>MLSRKGIIPEEYVLTRLAEDPAEPRYRTRERRARFVSKKGNCNVAHKNIREQGRFLQDVFTTLVDLKWPHTLLIFTMSFLCSWLLFAMVWWLIAFAHGDLAPGEGTNVPCVTSIHSFSSAFLFSIEVQVTIGFGGRMVTEECPLAILILIVQNIVGLMINAIMLGCIFMKTAQAHRRAETLIFSKHAVITLRHGRLCFMLRVGDLRKSMIISATIHMQVVRKTTSPEGEVVPLHQVDIPMENGVGGNGIFLVAPLIIYHVIDSNSPLYDLAPSDLHHHQDLEIIVILEGVVETTGITTQARTSYLADEILWGQRFVPIVAEEDGRYSVDYSKFGNTIKVPTPLCTARQLDEDRSLLDALTLASSRGPLRKRSVAVAKAKPKFSISPDSLS[4x];>MPLAFCGTENHSAAYRVDQGVLNNGCFVDALNVVPHVFLLFITFPILFIGWGSQSSKVHIHHSTWLHFPGHNLRWILTFILLFVLVCEIAEGILSDGVTESRHLHLYMPAGMAFMAAITSVVYYHNIETSNFPKLLIALLIYWTLAFITKTIKFVKFYDHAIGFSQLRFCLTGLLVILYGMLLLVEVNVIRVRRYIFFKTPREVKPPEDLQDLGVRFLQPFVNLLSKGTYWWMNAFIKTAHKKPIDLRAIGKLPIAMRALTNYQRLCVAFDAQARKDTQSPQGARAIWRALCHAFGRRLILSSTFRILADLLGFAGPLCIFGIVDHLGKENHVFQPKTQFLGVYFVSSQEFLGNAYVLAVLLFLALLLQRTFLQASYYVAIETGINLRGAIQTKIYNKIMHLSTSNLSMGEMTAGQICNLVAIDTNQLMWFFFLCPNLWAMPVQIIVGVILLYYILGVSALIGAAVIILLAPVQYFVATKLSQAQRSTLEHSNERLKQTNEMLRGMKLLKLYAWESIFCSRVEVTRRKEMTSLRAFAVYTSISIFMNTAIPIAAVLITFVGHVSFFKESDLSPSVAFASLSLFHILVTPLFLLSSVVRSTVKALVSVQKLSEFLSSAEIREEQCAPREPAPQGQAGKYQAVPLKVVNRKRPAREEVRDLLGPLQRLAPSMDGDADNFCVQIIGGFFTWTPDGIPTLSNITIRIPRGQLTMIVGQVGCGKSSLLLATLGEMQKVSGAVFWNSNLPDSEGEDPSSPERETAAGSDIRSRGPVAYASQKPWLLNATVEENITFESPFNKQRYKMVIEACSLQPDIDILPHGDQTQIGERGINLSGGQRQRISVARALYQQTNVVFLDDPFSALDVHLSDHLMQAGILELLRDDKRTVVLVTHKLQYLPHADWIIAMKDGTIQREGTLKDFQRSECQLFEHWKTLMNRQDQELEKETVMERKASEPSQGLPRAMSSRDGLLLDEEEEEEEAAESEEDDNLSSVLHQRAKIPWRACTKYLSSAGILLLSLLVFSQLLKHMVLVAIDYWLAKWTDSALVLSPAARNCSLSQECDLDQSVYAMVFTLLCSLGIVLCLVTSVTVEWTGLKVAKRLHRSLLNRIILAPMRFFETTPLGSILNRFSSDCNTIDQHIPSTLECLSRSTLLCVSALTVISYVTPVFLVALLPLAVVCYFIQKYFRVASRDLQQLDDTTQLPLLSHFAETVEGLTTIRAFRYEARFQQKLLEYTDSNNIASLFLTAANRWLEVRMEYIGACVVLIAAATSISNSLHRELSAGLVGLGLTYALMVSNYLNWMVRNLADMEIQLGAVKRIHALLKTEAESYEGLLAPSLIPKNWPDQGKIQIQNLSVRYDSSLKPVLKHVNALISPGQKIGICGRTGSGKSSFSLAFFRMVDMFEGRIIIDGIDIAKLPLHTLRSRLSIILQDPVLFSGTIRFNLDPEKKCSDSTLWEALEIAQLKLVVKALPGGLDAIITEGGENFSQGQRQLFCLARAFVRKTSIFIMDEATASIDMATENILQKVVMTAFADRTVVTIAHRVHTILSADLVMVLKRGAILEFDKPETLLSQKDSVFASFVRADK[4x]

ATP-sensitive potassium channels (KATP) are ion channels that selectively allow potassium ions to permeate the cell. Specifically, they are inhibited by ATP and activated by Mg-ADP. Previous studies have established that the functional KATP channel is a hetero-octamer composed of four inward-rectifying potassium channel 6 (Kir6) subunits and four sulfonylurea receptor (SUR) regulatory subunits. KATP channels in pancreatic islets are composed of Kir6.2 channel subunits and SUR1 regulatory subunits.

The third structure is the KATP channel in complex with Mg-ADP, VO43-, PIP2 and NN414, a ligand combination that favors the NBD-dimerized state of SUR1, which is solved to 4.3 Å (abbreviated, Mg-ADP state). We observed similar “T state” and “R state” conformational heterogeneity of the Kir6.2 CTD and SUR1 ABC transporter module as in the ATP + GBM state or the ATP state. Here, we refer to class 1 structure as the “T state” (the tense state) and class 2 as the “R state” (the relaxed state). Similarly to the ATP or ATP + GBM state, the CTD of Kir6.2 in “T state” has a clockwise rotation (~11.8°) relative to that of “R state”. Moreover, the ATP binding sites of Kir6.2 are also occupied by ADP molecules, and the Kir6.2 channel is in the closed conformation, similarly to the ATP + GBM state, which is consistent with the result that ADP can inhibit the KATP channel albeit at a lower affinity. The ADP binding mode at the inhibitory site of Kir6.2 is similar to that of ATP or ATPγS. Because ADP lacks the γ phosphate, there is no direct interaction between ADP and the γ-phosphate-coordinating residue R50. This explains why ADP binds Kir6.2 with a lower affinity and the R50 mutation shifts the IC50 curve to a similar range of ADPβS on wild-type channels. We did not observe any density at the PIP2 binding site, probably due to the low affinity of the 08:0 PI(4,5)P2 to the purified protein and also the negative cooperativity of inhibitory nucleotide binding and PIP2 binding on Kir6.2.1-[2-(trifluoromethyloxy)phenyl]thiourea | C8 H7 F3 N2 O S | 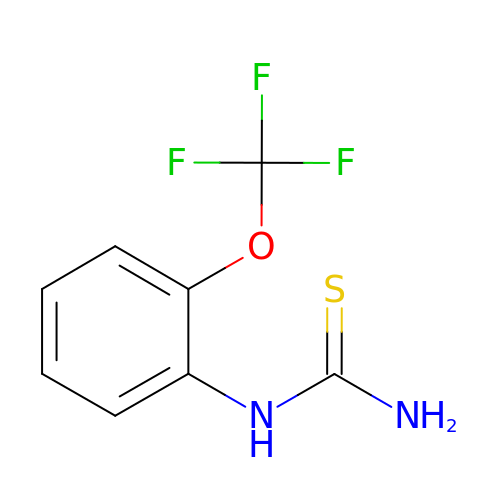HYKOSRYWIURWQI-UHFFFAOYSA-N>NESVRYDATFP[2x];>GSLIGLMKDAFQPHHHHHHHLSPHPPGTVDKKMVEKCWKLMDKVVRLCQNPKLALKNSPPYILDLLPDTYQHLRTILSRYEGKMETLGENEYFRVFMENLMKKTKQTISLFKEGKERMYEENSQPRRNLTKLSLIFSHMLAELKGIFPSGLFQGDTFRITKADAAEFWRKAFGEKTIVPWKSFRQALHEVHPISSGLEAMALKSTIDLTCNDYISVFEFDIFTRLFQPWSSLLRNWNSLAVTHPGYMAFLTYDEVKARLQKFIHKPGSYIFRLSCTRLGQWAIGYVTADGNILQTIPHNKPLFQALIDGFREGFYLFPDGRNQNPDLTG[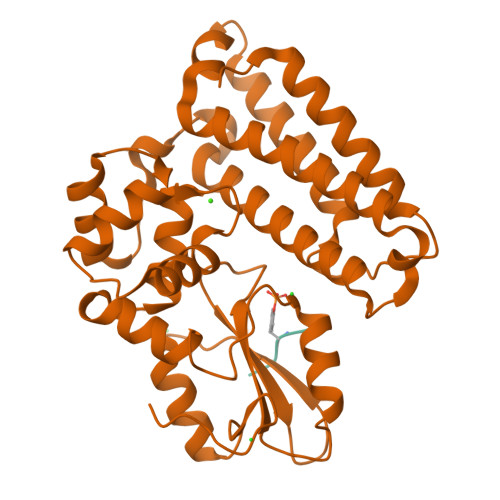2x]> MALKKAPKLFKTFFHWKLWKFSIIVFVFLVFLFLLQREVGVQDFKDEAGIEPVVGKKSHVLGLVLNAMNNIKGAKPKMQIKAP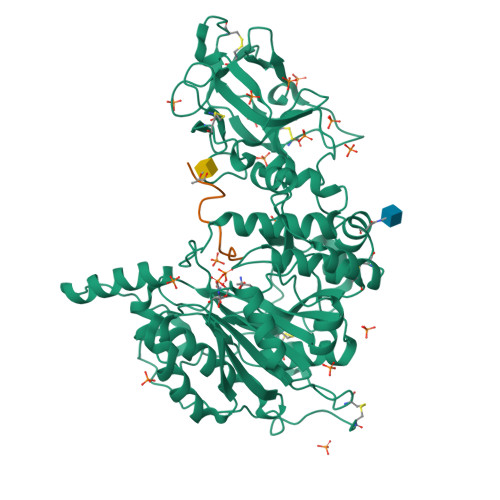IRQTKVPGERHCLPGHYTPVELKPFLDRPLQDPNAPGASGKAFKTINLNSEEQKEKQAGEEKHCFNAFASDRISLHRDLGPDTRPPECIEQKFKRCPPLPTTSIIIVFHNEAWSTLLRTVHSVMYTSPAILLKEIILVDDASVDEYLHDKLDEYVKQFQIVKVVRQKERKGLITARLLGASVATGETLTFLDAHCECFYGWLEPLLARIAENPVAVVSPDIASIDLNTFEFSKPSPYGHSHNRGNFDWSLSFGWESLPKHENKRRKDETYPIRTPTFAGGLFSISKDYFEYIGSYDEEMEIWGGENIEMSFRVWQCGGQLEIMPCSVVGHVFRSKSPHTFPKGTQVITRNQVRLAEVWMDEYKEIFYRRNTEAAKIVKQKTFGDISKRIDLRQRLQCKNFTWYLSNVYPEAYVPDLNPLFSGYLKNIGNRMCLDVGENNHGGKPLIMYSCHGLGGNQYFEYSAHHEIRHNIQKELCLHASKGPVQLRECTYKGQKTFAVGEEQWLHQKDQTLYNEALHMCLTGNGEHPSLASCNPSDPFQKWIFGQND;> ATGAGAGAGTTPGP>[6x]MKPTHWGAALALAAACFTTSAYALEYPIGTPQNLAGMEIAAVYLQPIDMEPEGHMRKASESDIHIEADIHALSNNPNGYPEGFWVPFLFIKYEITKVGGSGAPITGDMMAMVASDGP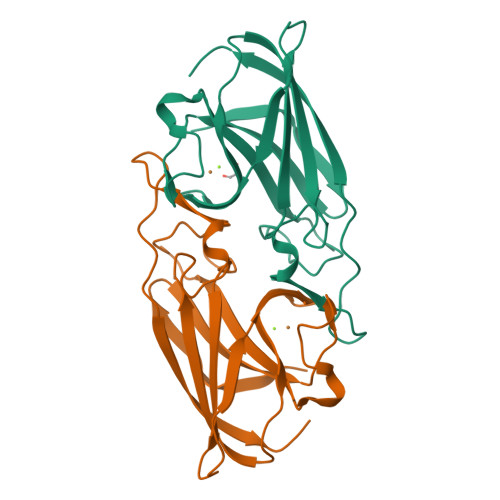HYGDNVKLQGPGKYKVKYTIYPPNAKENPMSPYYGRHTDRETGVRPWFKTFSVEWDFTYAGIGKKGGYSWSHPQFEK>[14x]MRKENELLRREKDLKEEEYVFESPKMKEILEKIKKISCAECPVLITGESGVGKEVVARLIHKLSDRSKEPFVALNVASIPRDIFEAELFGYEKGAFTGAVSSKEGFFELADGGTLFLDEIGELSLEAQAKLLRVIESGKFYRLGGRKEIEVNVRILAATNRNIKELVKEGKFREDLYYRLGVIEIEIPPLRERKEDIIPLANHFLKK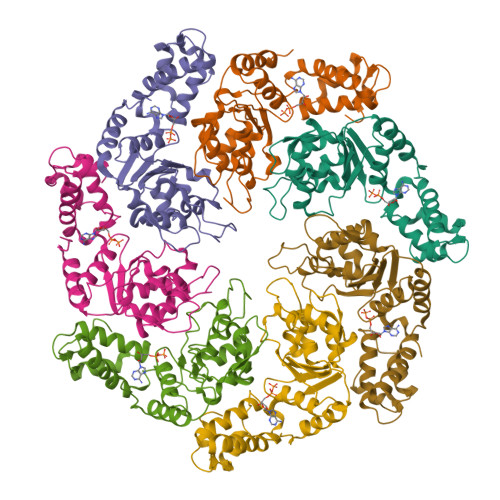FSRKYAKEVEGFTKSAQELLLSYPWYGNVRELKNVIERAVLFSEGKFIDRGELSCLVNSK> 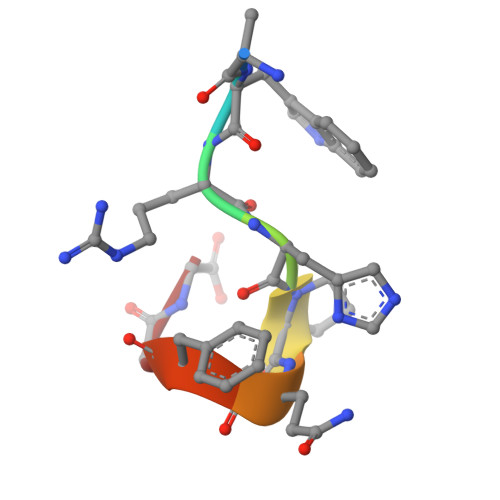AWRHPQFGG>[2x]MAFSGSQAPYLSPAVPFSGTIQGGLQDGLQITVNGTVLSSSGTRFAVNFQTGFSGNDIAFHFNPRFEDGGYVVCNTRQNGSWGPEERKTHMPFQKGMPFDLCFLVQSSDFKVMVNGILFV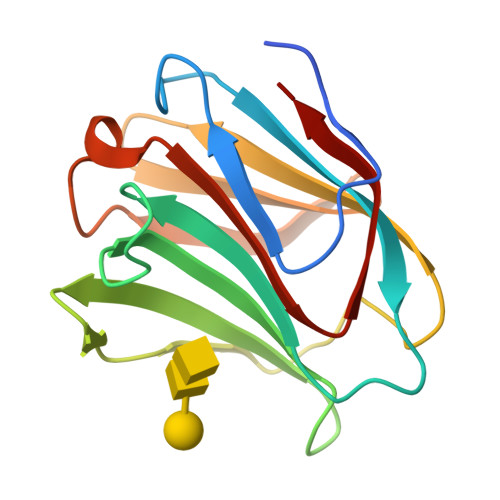QYFHRVPFHRVDTISVNGSVQLSYISFQ>MKGSEEAYLVSDKATKMYSLTKDSEKNHPSKPPLQDEENPQSKYHCHNNNKKAYDARQREQTFAKKKLCIASLICFVFISAEIVGGYIAGSLAVVTDAAHLLVDLSSFFISLCSLWLSSKSSTTRLTFGWHRAEILGALMSVITIWLVTGVLVYLACERLIRPDYTIDGTVMLITSACALGANLVLALILHQSGHGHSHAGGKHEHMASEYKPQTNASIRAAFIHVIGDLFQSISVLISALIIYFKPEYKMADPICTFIFSIFVLITTVTVLRDLLTVLMEGTPRGIHYSDVKQSILAVDGVKSVHSLHLWALTMNQVILSAHIATDIVGESKRILKDVTQNVFARFPFHSVTIQVEPIEDQSPECM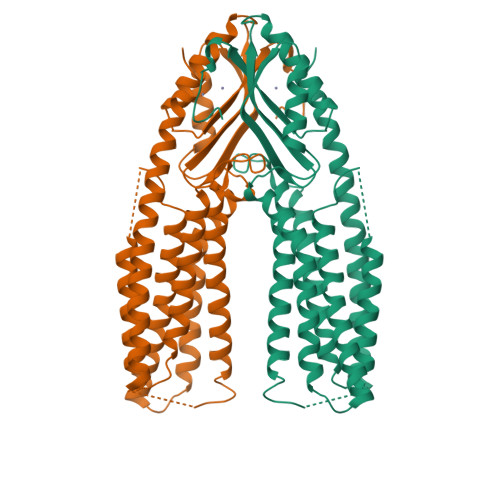FCYEPTQ[2x]>[2x]GPEFSMEDLIPLVNRLQDAFSAIGQNADLDLPQIAVVGGQSAGKSSVLENFVGRDFLPRGSGIVTRRPLVLQLVNATTEYAEFLHCKGKKFTDFEEVRLEIEAETDRVTGTNKGISPVPINLRVYSPHVLNLTLVDLPGMTKVPVGDQPPDIEFQIRDMLMQFVTKENCLILAVSPANSDLANSDALKVAKEVDPQ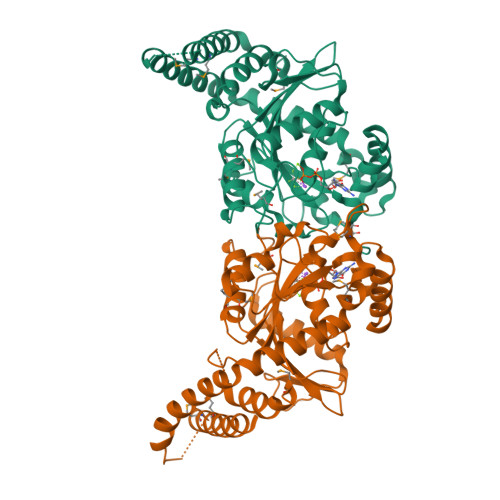GQRTIGVITKLDLMDEGTDARDVLENKLLPLRRGYIGVVNRSQKDIDGKKDITAALAAERKFFLSHPSYRHLADRMGTPYLQKVLNQQLTNHIRDTLPGLRNKLQSQLLSIEKEVEEYKNFRPDKHGTDSRVDEMLRMYHALKEALSIIGNINTTTV> QRTKIVVKVHMPCGKSRAKALALAASVNGVDSVEITGE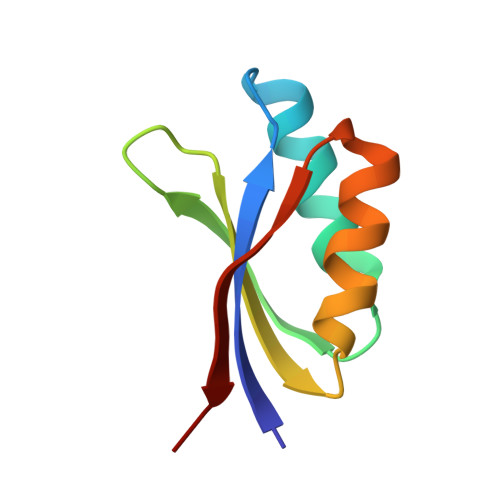DKDRLVVVGRGIDPVRLVALLREKCGLAELLMVELVK>[8x]MAVPEVVVEGVVFPPVARPPGSAGSHFLGGAGVRGIEIGGNFIKFTAIGVYLEDAA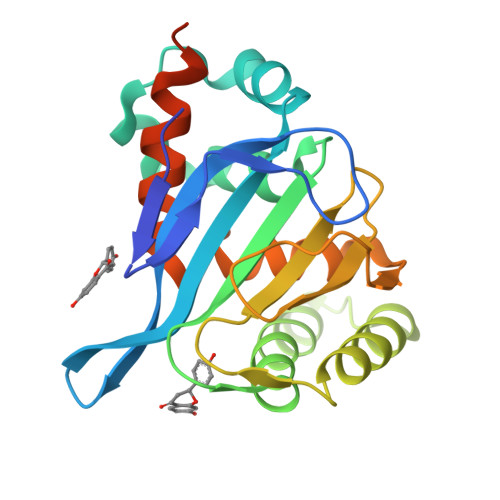VSALAKKWAGKTADELASDAAFFRDVVTGDFEKFTRVTMLLPLTGEQYAGKVTENCVAFWKAVGLYTDAEGVAVEKFKEAFKPETFPPGASILFTHSSTGVLTVAFSKDSSVPASGGVAIENKHLCEAVLESIIGEHGVSPAAKLSLAARVSELLTKGTAGAADAPQAEPVSVTA>[2x]TSSINFLTSDDDASAAAMEAFIGTNHHSSLFPPPPQQPPQPQFNEDTLQQRLQALIESAGENWTYAIFWQISHDFDSSTGD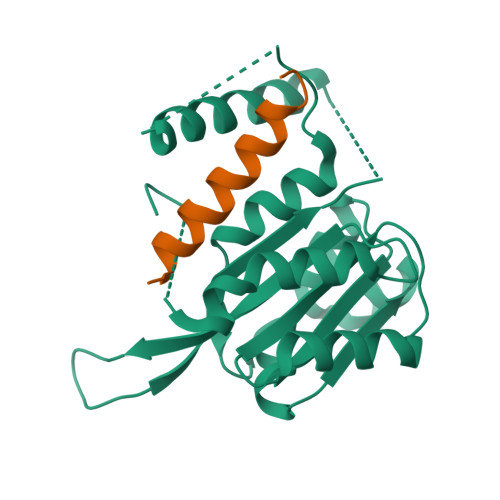NTVILGWGDGYYKGEEDKEKKKNNTNTAEQEHRKRVIRELNSLISGGIGVSDESNDEEVTDTEWFFLVSMTQSFVNGVGLPGESFLNSRVIWLSGSGALTGSGCERAGQGQIYGLKTMVCIATQNGVVELGSSEVISQSSDLMHKVNNLFNFNNGGG;>[2x]SVPQARKASLARFLEKRKERLM(1R,4aS,7S,8aR)-1,4a-dimethyl-7-(prop-1-en-2-yl)decahydroquinolinium 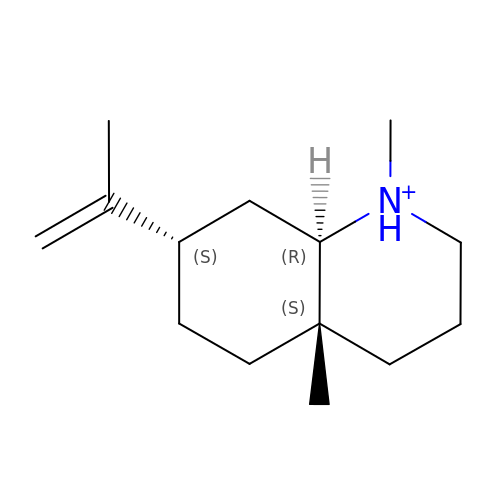| C14 H26 N | HQXXDILNZLFDML-BFHYXJOUSA-O Plectasin consists of 40 amino acids and shows well-defined secondary structural elements in form of an α-helix (M13-S21) and an antiparallel β-sheet (G28-A31; V36-C39). The structure of plectasin is stabilized by three disulfide bridges (C4-C30; C15-C37; C19-C39), which is typical for this type of defensins and leads to high conformational stability. Plectasin contains a cysteine-stabilised α-helix-β-sheet structure, which remains intact upon fibril formation. We have determined the structure, kinetics, and functionality associated with the pH-responsive self-assembly of the enhanced plectasin variant PPI42 into helical protein fibrils.

To elucidate the structural features that allow PPI42 to assemble into fibrils, while the plectasin wildtype did not fibrillate, we determined the crystal structure of the plectasin wildtype at a resolution of 1.1 Å. Our plectasin wildtype structure shows a high similarity to the published crystal structure (PDBID: 3E7U69) with only minor differences in the N-terminal loop (all-atom RMSD: 0.316 Å). When we compared our wildtype plectasin crystal structure to the fibril cryo-EM structure of PPI42, we observed a significant structural difference in the N-terminal loop region between amino acids 9 and 14. Two of these  positions are mutated in PPI42 (D9S; Q14K). We observed a network of polar interactions in the plectasin wildtype with (D9) forming a salt bridge to (N5). When mutated to (S9) in PPI42, the sidechain orientation changes and the sidechain forms a hydrogen bond to the (G6) backbone, which disrupts the network stabilizing this part of the N-terminal loop. In the plectasin wildtype, (H18) is coordinated in two different ways (50/50% distribution) stabilized by polar interaction with (Q14) and π-stacking with (F2), while in PPI42 only the π-stacking with (F2) occurs due to the mutation Q14K. Notably, the sidechains of (E10), (D11), and (D12) form intermolecular interfaces both in the protein crystal of the wildtype and in the fibril of PPI42. However, their orientation differs significantly between wildtype and PPI42. This structural difference may contribute to the different arrangement with the mutant forming the fibril and the wildtype forming the crystal.

> GFGCNGPWDEDDMQCHNHCKSIKGYKGGYCAKGGFVCKCY> MEKDGLCRA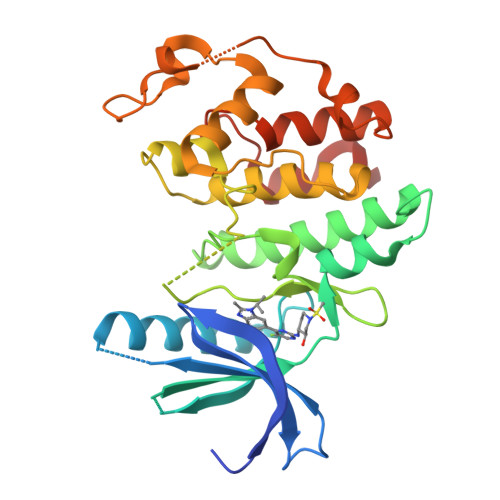DQQYECVAEIGVGAYGTVFKARDLKNGGRFVALKRVRVQTGEEGMPLSTIREVAVLRHLETFEHPNVVRLFDVCTVSRTDRETKLTLVFEHVDQDLRTYLDKVPEPGVPTETIKDMMFQLLRGLDFLHSHRVVHRDLKPENILVTSSGQIKLADFGLARIYSFQMALTSVVVTLWYRAPEVLLQSSYATPVDLWSVGCIFAEMFRRKPLFRGSSDVDQLGKILDVIGLPGEEDWPRDVALPRQAFHSKSAQPIEKFVTDIDELGKDLLLKCLTFNPAKRISAYSALSHPYFQHHHHHH> MQNALKVGFWPAYSVSEFPPSKINSRLFTHLYYAFAELNAPTFEVRVPPGSEKTAEDFTPTVRRLNPSVKTLISIGGWGSEVRDNFAKL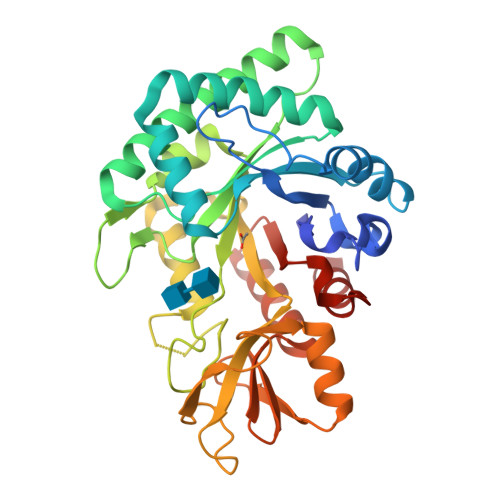NSDASARQRFVKSSIALARRYGFHGLDLDYQYPEPQLEMENFVKLVSELTAAIREEARTSGKPRLLLTEAVYFHQKLFPWEVVTEYPVQFIAAGLDWVNVMAYDFHGSWENFTGAPAALRDPNSKFTASVGIESFLAAGMPPEKLVLGIPLFGRSWLLKNNNEVGIGAPAVGAGPVDGALSFSEIQNFIRGGAREVFDTTTVSAYAYKDNVWVGYDNQQSVALKVQYAKEKRLGGYFFWSVNQDIDAILPKIASDTWGG> GPGSEFSLDHSDLVAELLKELSNHNERVEERKIALYELMKLTQEESFSVWDEHF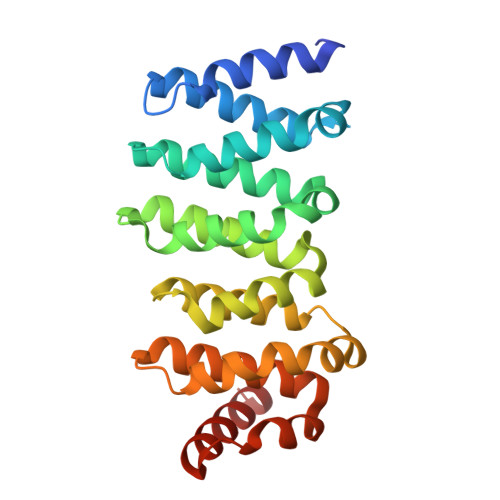KTILLLLLETLGDKEPTIRALALKVLREILRHQPARFKNYAELTVMKTLEAHKDPHKEVVRSAEEAASVLATSISPEQCIKVLCPIIQTADYPINLAAIKMQTKVIERVSKETLNLLLPEIMPGLIQGYDNSESSVRKACVFCLVAVHAVIGDELKPHLSQLTGSKMKLLNLYIKRAQTGS>[3x]MRRFGSKFASGLASRCALACPLASAATAPAGASTTSSTSSAQKSFFKTTEMIGYVHSIDGTIATLIPAPGNPGVAYNTIIQIQVSPTTFAAGLVFNLEKDGRIGIILMDNITEVQSGQKVMATGQLLHIPVGAGVLGKVVNPLGHEVPVGLVTRSRRLLDSTLGKVDTGAPNIVSRSPVNYNLLTGFKAVDTMIPIGRGQRELIVGDRQTGKTSIAVSTIINQVRINQQILSKNAVISIYVSIGQRCSNVARIHRLLQSYGALRYTTVMAATAAEPAGLQYLAPYAGVTMGEYFMNRGRHCLCVYDDLSKQAVAYRQISLLLRRPPGREAYPGDVFYLHSRLLERAAMLSPGKGGGSVTALPIVETLSNDVTAYIVTNVISITDGQIYLDTKLFTGGQRPAVNIGLSVSRVGSSAQNAAMKGVAGKLKGILAEYRKLAADSVGGQQVQTIPMIRGARFVALFNQKQPSYFMNAIVSLYACLNGYLDDVKVQYVKFYEYLLVHRDLGIMYGTAKNKFFYMYVQELNYLIRFFTLNSPILHGELEEMLKQHTHLFLQHYQSKMNAIKSEKDVKALKNLLYSCKRAV;>MLTRFRSAVLRGAVSITGARAASTAPVADHKGRVGHVSQVIGAVVDVHFADGVPPVLTALDVVDKLGRDEPLTLEIVQHLDAHTGRCIAMQTTDLLKLKAKVVSTGGNISVPVGRETLGRIFNVLGDAIDQRGPVGEKLRMPIHAVAPKLADQAAEDAVLTTGIKVIDLILPYCKGGKIGLFGGAGVGKTVIIMELINNVAKGHGGFSVFAGVGERTREGTDLYLEMMQSKVIDLKGESKCVLVYGQMNEPPGARARVAQSALTMAEYFRDVEGQDVLLFIDNIFRFTQANSEVSALLGRIPAAVGYQPTLAEDLGQLQERITSTTKGSITSVQAVYVPADDITDPAPATTFSHLDATTVLDRAVAESGIYPAVNPLECASRIMDPDVISVDHYNVAQDVVQMLTKYRELQDIIAVLGIDELSEEDKLIVDRARKLVKFLSQPFQVAEVFTGMTGHYVQLDDTIDSFSGLLMGTYDQVPEMAFYMVGGINSVLEKAKKMAEEAAELEKMRRARVAQASS[3x];> MSGKLRLYKEKLEGYNRFYSIVKTIKMVTLAKYRAAQGRIRTRDFSLRYTELAFSKPQASRDAVVAAKNALVYIPITTNRGSCGALNSNIVRCIDSVVSSKMVLMPVGKRGIDSFSKLYPDEFRYGIINDMKESMHFGYATFVIENAYEVSKDADRYQVIFNRFVSAGVQRNAVYNIPSYEKWKEDLADAASSDNQKNRYLFANALQNEEEQLIRDFFDFHAALAVLNAVGENELSEQAARLVAVEGQLTNISSLQQRTSSLYNKTRQFGITAALIEILSAMSSLEGNAMKGVRRNKFWEGAVTK;> MFRTFGRRLVSCTLPLLQSAPHDLPEGFEFMEHKVVNKDIHAPHENLETLRLTLTRQDEFLLREEPVKCVTVTGTNGEYGIYPGHAYKIVQLNPSPLTVEYTDGTTKKYFVSGGFAHINNEGSCDVNTVECTLLDDLDLAIAEKELAAQQAALGSAKDDKAKSVVEIRISVIEAVIAALKHH;> MIRRSCALLSSSWRDHGISYLKYLNVCTETLHSTVKESRRAKYERWSKPCYTAQRPDGAGGQETIDKVPIHTKDY;>[3x]MMRRVYSPVFCSVAAARFAATSAAKKYDLFGYEVDTNTAPWIEKIKKCKYYDEAGEVLVNMNVSNCPPDIATYNATLQCIYQSPSKQSTPVDNESKFCAMMDLLEEMQHRNRLKPNEESWTWVMKECVKSGQFRLGYCIQQVMETECKGCPADLVKANEANAQKAKTEGKEHPGHLSQQAGLFDVKVE;>MSAKAAPKTLHQVRNVAYFFAAWLGVQKGYIEKSANDRLWVEHQRKVRQQNVERQQALDSIKLMQQGVRATTPGQLEGVPAELQQLAEAFTK[2x];>[2x]MSSTKCAVACKIMTPLCNAASKVQARSAKKLAALTDAGIQKTISEHNANGTDAAVSSTKRYLAEQRQLFHYRVVRFFDECHYIISGEYFAQYTKVNLIWDLRFLTKLVVLFLIGTVLGRQSIFPPIDPDSPLVEALVTKVNPNY;> MFRRLSSSARAVVAARFYTPPEGLKKLYASDFENSKYPLNIVPSDSVLFAKFLYKAAEEKGNFDNILSDFQKIAAAASKLPIFWERTAVVEKIPEFKQLSEPTFFTLVWMQNNGMLELIQEVAEVYETFVNAKQKKAVAKIFVAPGGEKNVEEARRVAEELHKGLKELADYTLVLKTVVDRTIVKGFAVELAGQYVNKAEGQQKQAGRADEVDYTNLPAPKPQKTVWDDNIETEVLRKYLDGLSQYDMEEAKYGV;>MMRRLALQSSIRRATPFATPLVASTKALNPMCSAITIREASTVAISVQGLHYVGTGLAAIALAGVGLGIGTIFGNLLVACARQPNLTKMLFNYAILGFALTEAIGLFALMLAFLMLFS[10x];> MFLFFFCDLFWLRLLLCMYYCVWSRLCFIVYFNCLMLIFDFLLFCLFDLYLFVGLCLFLLLWFMLFNLYSLILYYCITYLNLYLLFCIVFLLYIAFLFLFCFLCDFFLFNNLLVGDSFMDVFFIRFLLCFLECFSLLCRCLSTFLRLFCNLLSSHFLLLMFFDFFYFIFVFFFYGVFCYWFILFIFVFCFCLLFYVFLYLLDLFAAILQLFIFCNMILQLIMDFLLFLLFV;> MLRRLGANVSNMARPMNKYAVTVSPRRHLEPMSTWYLASWAMVWYYAFFFWMPMVWTDIMVPSFVYNKLPVIHFLQEKRAEQKLRRVLDETYTEWTEELDQAHVTDAITRSLNI;> MRRVSSPNITIQSVRWISGVSPLLYFPPTTTSTTNREDQINKNTNIAIQMIKRYKGEVPPHYTRKSSATIEQVEKEIDALLGGAEKLRKTSTDDQPMDKLTLMERCLRHALWSYHKEEGRYDFDQIGRWVVYTPEDEVKLAQLKREVEAKEKLAALRKRREEEGLPGGPVPRINWPQEYSSFIDREPVVAKRIRYDTLASTTLERDEKQIESTLQQYRRASQDKRLDDLVDLLERFKPVLAREAIMQRLTIKHLEGQLGVWRYMDWCPEVRDRAELEVDITGWQWWSPLEERRLLPVRLRSVNEVREIMSKTQAKKSAEAAERNPIVTQTSTGDNARDRLLKEVLALQARINQRDEVEPSQTEQKKKAHH;> MQGSWSVLKKNCSNFFPGLLAFAQQTQEAYGIWLRIYNRQQKYGPTDFVEQSETFSPDYHKRFHSQDKNMWVDKELCTEVSQKEVARLMTYKLDMWRMAHCAGALLATGGYAIPFGLFWLANDTWVPSSFNLTGEELRAWREAQDLYRYRSAPSYLTDTKWHFDFHAYPWNETQERAWDDLFEKNDVRRDPKVVRPAAEMYDGFIKFELIRRKSLRHLCRSMNIPTFPMLARLCNGTRVRDYWNLAWCEDYMVITQRLHESMTDEELYDYAWRRYLAPYDKNLNREQLMERVEDYFEFLGPDFVAHGKAPNLVILTNYVLGYYNDPAYLEGDISELDKNDYDHLASWGKDAFLRRLEFENGPLRDQVEAHTQRLLAERAAIAKGDNAAAVEGRHTA;> MVLFSTYRSSRLVSKEFLHGPVMRFRALGEYYFQRAWNGTLNWALPGEYRLYAVMIPFIYFYHRWHNDHTLDRDHVEKAMIMRWGGTLEDVRKLSAKDQLRVRCFTDIEKLYSAYGPKDTYLQPPGDTLPGKDFYRKAGGAQAHH;> MSKQLTFISAGATAAVLQSASAIVSKVAGGRVQTKTAKEAGRHAVVVGPETPIGVHTAVTEVPKSAQDPLFSGVSTVVVRAVLPRAAPDSVQLRDALDVYASAGIDTKEEVRSATEAFKKSAEVAVGKAKAKGVKRIVLVVKQASKHNCINELFKKISTETIESAGLTTEVVGTAAVANQLIVNPESLGVVLLNDVAATEQIELAFAGVVGGVSRVYHTVEGGKISAGHSFKSVALAVAQELRELGLSSEADKVEAAASKNPRAVVSAL;> MRRTFISFSAASAAAAAPVTSTKMQTLHKLLTGEVSFKNKAPVKDCNIVHQFGENWATELSAYAKTLPAEQQKIIVRQIARVKLTRYTVAELAAYCGDGPALLDETARAANIEQGVAFVKAKGVEAFEKYVAEESTNANWKPEEAKKFIEDVKAKAK;> MVYTRWKCDRLPVFQLKLFTQEYPMHAAVGIFTIIFLWKHMSHCSEETERKYGWWAGYPYWRDPIARRNETKYKQMIINNDVDITHPKWTGCSVEQLEELSRVV;> MTKYELKMQYFDEWMIRWRKFQTESDWEIEKGRQWWRRFNMAVSGALFCGLVLYTSGTATLKRQYGLPHFFDIGVDGQAKETMLKTLTSRWRYTPQGYGRVLITGVPTYILFVTLEHYRERRRMQQYLQQNTVFGEQMRRLLSTGKIEEYLPVNIKATLPASQQAIYNY;> MLRRSSAALIRRTPVRHSGGELFVRPKLEEIPPADQCRGFFGPLNDSLKFLRLLDIKWMMNRAVAMRREYLIATPTLFTFIWMFTWKGAVIYFWGDRAPPRRMDWNTEETGRLPLGFKPTPAPL;> MLRKTPLFAMATTRKALVGNGPTFSTGGECMNTCDIQNAFPMNDRGVRSSSPFQEPNTAIYDSYLAWTYFQPMDVHIEKLPAPEAKYYQRHTKKPWDVSSTELTEIQSRKKYFQTLGYLVAFIYLYFLMPKEKSFSGLSGPDGHWIMLPKGRPELF;> MSSGFHFHDVSNDAIKGMPPSEALHKHLENAQLAHRICLAKALKAGEPPVEKCALTWGEVLIRYQAWSEYRPPFQDSVAQAKYKKYWSKKRQEEDDKNPFK;> MLRRLVPRVMMAPMGGATALCTSRGYNMLVFRDPKRRPQLSEEERAKVVVNQAEWPEEFKDFDPDDPYKNSPEIIKGMSSWNLFLWGVECAFIYQFYELVFPKSI;> MTENIEAVMSDFWSNPADHFRPNLKALTLYAERQHYVDRWLHVKERWLAPWYLPWWSPLFQLGTWYSQRSRNLFLVENHLSYRPYKFRRNDEDRNNPY;> MLLGGFVPRRFSQFNRDPCWMFFIFSVGFWLGEYPAMMIKYNARDLVYDPHRYVWSHHDDHH

Mitochondrial ATP synthase consists of the soluble F1 and membrane-bound Fo subcomplexes and occurs in dimers that assemble into oligomers to induce the formation of inner-membrane folds, called cristae. Dissociation of ATP synthase dimers into monomers results in the loss of native cristae architecture and impairs mitochondrial function. Here, we report cryo-EM structures of the intact ATP synthase dimer from Trypanosoma brucei in ten different rotational states. Although overall dimer architecture varies among eukaryotes, we find that subunit-g together with subunit-e form an ancestral oligomerization motif, which is shared between the trypanosomal and mammalian lineages.

To describe the conformational space of the T. brucei ATP synthase, we resolved ten distinct rotary substates, which were refined to 3.5–4.3 Å resolution. The three main states (1–3) result from three ~120° rotation steps of the rotor relatively to the static Fo. We identified five (1a–1e), four (2a–2d), and one classes of the respective main states. Throughout all the identified substeps of the rotational state 1 (classes 1a to 1e) the rotor turns by ~33°, which corresponds approximately to the advancement by one subunit-c of the c10-ring. While rotating along with the rotor, the F1 headpiece lags behind, advancing by only ~13°. In all classes F1 is in a similar conformation, corresponding to the catalytic dwell, observed previously also in the crystal structure of T. brucei F1-ATPase13. In accordance with the ~120° rotation of the central stalk, the conformations and nucleotide occupancy of the catalytic interfaces of the individual αβ dimers differ between the main states, showing ADP and ATP in the “loose” and “tight” closed conformations, respectively, and empty nucleotide binding site in the “open” conformation.>[2x]GQFTGTGTGGDVFKVDLNEQFDRADMVWIGTASVLVWIMIPGVGLLYSGISRKKHALSLMWAALMAACVAAFQWFWWGYSLVFAHNGSVFLGTLQNFCLKDVLGAPSIVKTVPDILFCLYQGMFAAVTAILMAGAGCERARLGPMMVFLFIWLTVVYCPIAYWTWGGNGWLVSLGALDFAGGGPVHENSGFAALAYSLWLGKRHDPVAKGKVPKYKPHSVSSIVMGTIFLWFGWYGFNGGSTGNSSMRSWYACVNTNLAAATGGLTWMLVDWFRTGGKWSTVGLCMGAIAGLVGITPAAGYVPVYTSVIFGIVPAIICNFAVDLKDLLQIDDGMDVWALHGVGGFVGNFMTGLFAADYVAMIDGTEIDGGWMNHHWKQLGYQLAGSCAVAAWSFTVTSIILLAMDRIPFLRIRLHEDEEMLGTDLAQIGEYAYYADDDPETNPYVLEPIRS

structures of the Mep2 transceptors from S. cerevisiae and C. albicans. function as ammonium receptors/sensors in fungal development. a central channel for the transport of ammonium. non-phosphorylated, with channels that are closed on the cytoplasmic side.

different crystal forms to high resolution (up to 1.5 Å). sequence extends for two residues beyond Ser453. differences in the rest of the CTR.Proteins attached to the surface of group A and group B streptococcal human pathogens that contain tandemly arrayed Rib domains have been associated with invasive infections and proposed as potential vaccine candidates. Here, we study Rib domains from Rib, R28, and from a surface protein from Lactobacillus acidophilus. Together, these 5 structures of homologous Rib domains, and further sequence analyses, show Rib is an example of domain atrophy, a rare event in domain structural evolution involving the loss of core secondary structure elements, and also reveal the remarkable structural malleability of this domain family. The structure, molecular dynamics simulations, and small angle X-ray scattering of a Rib domain pair suggest tandemly arrayed domains are likely to form an elongated rod on the bacterial cell surface, thus suggesting a possible mechanism of immune evasion mediated through domain number variation.

Structures of single Rib domains with ∼38% sequence identity were solved: RibR (S. agalactiae Rib; amino acids 230 to 308) and R28N (S. pyogenes R28; amino acids 230 to 307). A 1.8-Å resolution structure of R28N was solved using the structure of RibR as a search model; the Cα root-mean-square deviation (rmsd) between RibR and R28N is 1.0 Å. RibS belongs to the “Rib” subfamily, giving a Cα rmsd value of 0.6 Å for superposition with both RibR and RibR28N, versus a Cα rmsd of 2.3 Å for RibL. As predicted, the Ig-fold D/E strands missing from RibR and R28N are also missing from RibS but are present in the RibL structure. Antibodies against, or intranasal immunization with, Rib conferred protection in animal models of GBS infection while antibodies to R28 conferred protection in an animal model of S. pyogenes infection. Cross-protective immunity has been observed on immunization with Rib and R28 against strains expressing the noncognate antigen.

>[2x]SGAMDKIKYSPEAKHRTVEQHAELDAKDSIANTDELPSNSTYNWKNGHKPDTSTSGEKDGIVEVHYPDGTVDDVNVKVTVTSKKT>MSTLEQTIGNTPLVKLQRMGPDNGSEVWLKLEGNNPAGSVKDRAALSMIVEAEKRGEIKPGDVLIEATSGNTGIALAMIAALKGYRMKLLMPDNMSQERRAAMRAYGAELILVTKEQGMEGARDLALEMANRGEGKLLDQFNNPDNPYAHYTTTGPEIWQQTGGRITHFVSSMGTTGTITGVSRFMREQSKPVTIVGLQPEEGS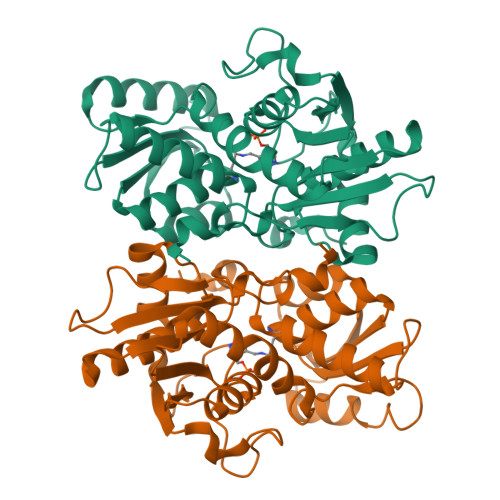SIPGIRRWPTEYLPGIFNASLVDEVLDIHQRDAENTMRELAVREGIFCGVSSGGAVAGALRVAKANPDAVVVAIICDRGDRYLSTGVFGEEHFSQGAGI[4x]>MAFNPPVIRAFSQPAFTYVFKFPYPQWKEKEWLLHALLAHGTEQSMIQLRNCAPHPDEDIIRDDLLISLEDRHFGAVLCKAVYMATTTLMSHKQRNMFPRCDIIVQSELGEKNLHCHIIVGGEGLSKRNAKSSCAQFYGLILAEIIQRCKSLLATRPFEPEEADIFHTLKKAEREAWGGVTGGNMQILQYRDRRGDLHAQTVDPLRFFKNYLLPKNRCISSYSKPDVCTSPDNWFILAEKTYSHTLINGLPLPEHYRKNYHATLDNEVIP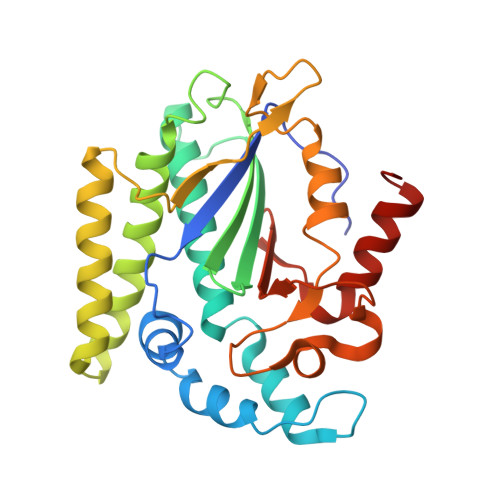G[2x]> MSQITIQARLISFESNRQQLWKLMADLNTPLINELLCQLGQHPDFEKWQQKGKLPSTVVSQLCQPLKTDPRFAGQPSRLYMSAIHIVDYIYKSWLAIQKRLQQQLDGKTRWLEMLNSDAELVELSGDTLEAIRVKAAEILAIAMPASESDSASPKGKKGKKEKKPSSSSPKRSLSKTLFDAYQETEDIKSRSAISYLLKNGCKLTDKEEDSEKFAKRRRQVEIQIQRLTEKLISRMPKGRDLTNAKWLETLLTATTTVAEDNAQAKRWQDILLTRSSSLPFPLVFETNEDMVWSKNQKGRLCVHFNGLSDLIFEVYCGNRQLHWFQRFLEDQQTKRKSKNQHSSGLFTLRNGHLVWLEGEGKGEPWNLHHLTLYCCVDNRLWTEEGTEIVRQEKADEITKFITNMKKKSDLSDTQQALIQRKQSTLTRINNSFERPSQPLYQGQSHILVGVSLGLEKPATVAVVDAIANKVLAYR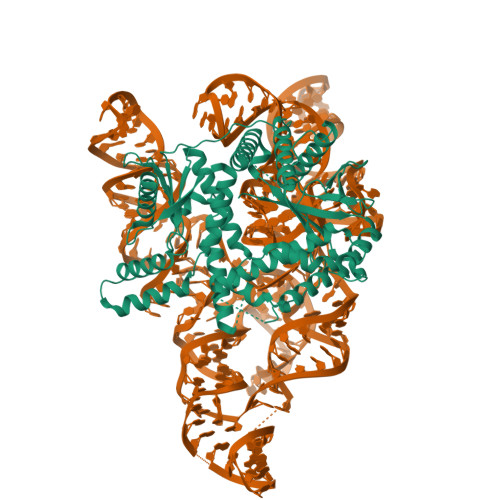SIKQLLGDNYELLNRQRRQQQYLSHERHKAQKNFSPNQFGASELGQHIDRLLAKAIVALARTYKAGSIVLPKLGDMREVVQSEIQAIAEQKFPGYIEGQQKYAKQYRVNVHRWSYGRLIQSIQSKAAQTGIVIEEGKQPIRGSPHDKAKELALSAYNLRLTRRS2,2',2''-[nitrilotris(methanediyl-1H-1,2,3-triazole-4,1-diyl)]triethanol | C15 H24 N10 O3 | 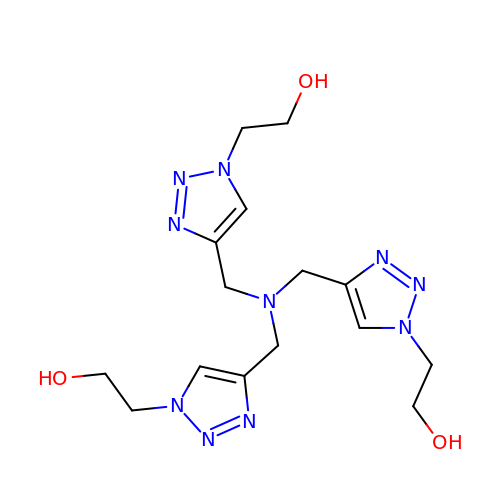UBECCOXTPTYDBC-UHFFFAOYSA-N>[2x]GSHMGGGGGIVLFVDFDYFYAQVEEVLNPSLKGKPVVVCVFSGRFEDSGAVATANYEARKFGVKAGIPIVEAKKILPNAVYLPMRKEVYQQVSSRIMNLLREYSEKIEIASIDEAYLDISDKVRDYREAYNLGLEIKNKILE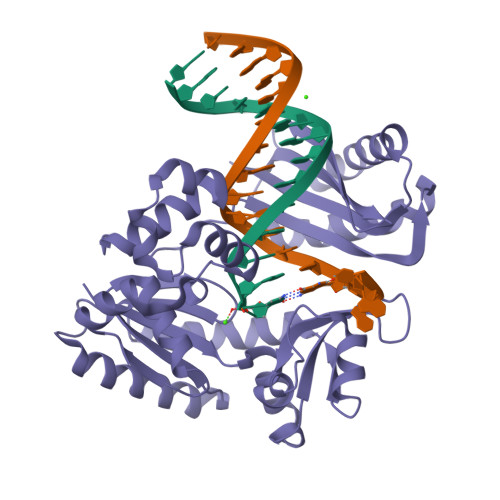KEKITVTVGISKNKVFAKIAADMAKPNGIKVIDDEEVKRLIRELDIADVPGIGNITAEKLKKLGINKLVDTLSIEFDKLKGMIGEAKAKYLISLARDEYNEPIRTRVRKSIGRIVTMKRNSRNLEEIKPYLFRAIEESYYKLDKRIPKAIHVVAVTEDLDIVSRGRTFPHGISKETAYSESVKLLQKILEEDERKIRRIGVRFSKFIEAIGLDKFFDT>GPGAGTVGGFIKRQQSKVVQNKVVYYGVGIWRGFMDGYQVHLEIENDIGQPPRLRNVTTNCQSSPWD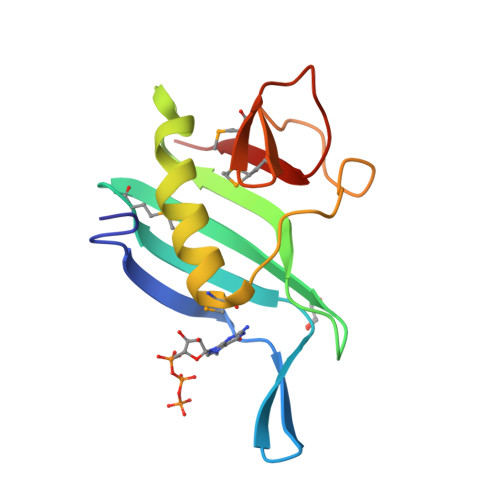LSIPIRQWAEDMGVTNNQDYSSKSSRGARYWMHSFRMQGPSKPFGCPVYIIK[2x]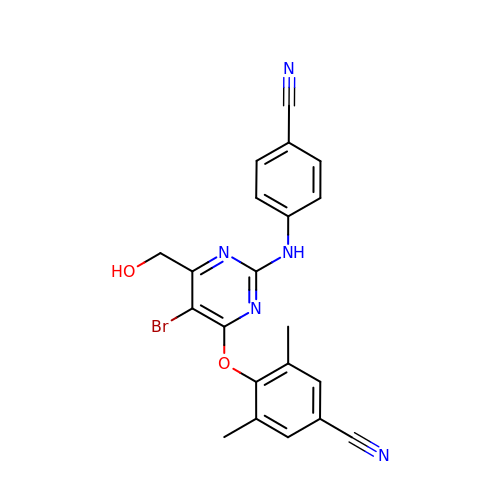(6-[4-(AMINOMETHYL)-2,6-DIMETHYLPHENOXY]-2-{[4-(AMINOMETHYL)PHENYL]AMINO}-5-BROMOPYRIMIDIN-4-YL)METHANOL | C21 H16 Br N5 O2 | LSIZSSASMKSUIU-UHFFFAOYSA-N>[2x]SNAMKKATMLTYLEEQLEKHLGDYEVGLDWDRKNHTIEVIVRLYAENNEQVAIDDVDG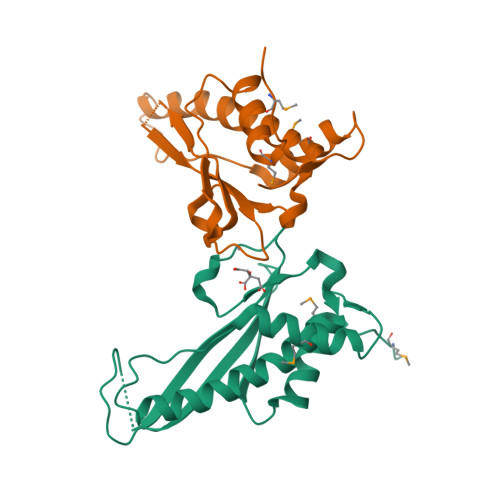TLSEEEFIEFEDGLLFYNPQKSVVDDEEYLVTIPYEGKKGLRKAVLDGFIHYLKVVLDEGQSDLLDFLSDETAEVFELHWEPADFEAMIKKVAETEKEQWIAYPSY> MLIAIEGVDGAGKRTLVEKLSGAFRAAGRSVATLAFPRYGQSVAADIAAEALHGEHGDLASSVYAMATLFALDRAGAVHTIQGLCRGYDVVILDRYVASNAAYSAARLHENAAGKAAA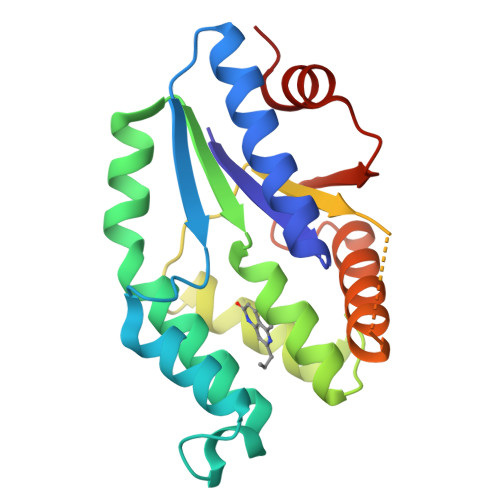WVQRIEFARLGLPKPDWQVLLAVSAELAGERSRGRAQRDPGRARDNYERDAELQQRTGAVYAELAAQGWGGRWLVVGADVDPGRLAATLAPP>[3x]STK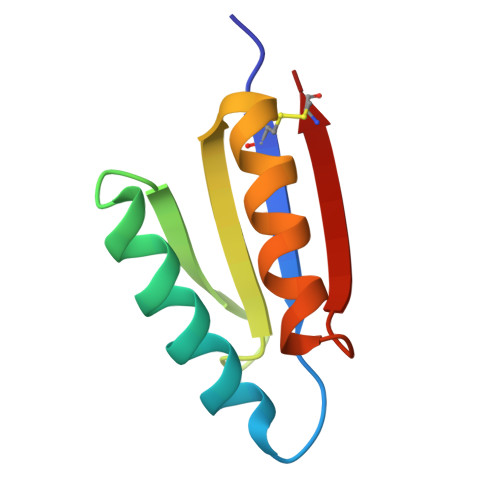CVVRFVFRGDLATLMLRAVKDHLKKEGPHWNITSTNNGAELVVRGIHESDAKRIAKWVEKRFPGVHTETQCD(5M)-5-{8-[({4-[(propan-2-yl)oxy]phenyl}methyl)amino]quinolin-4-yl}pyridine-2-carbonitrile | 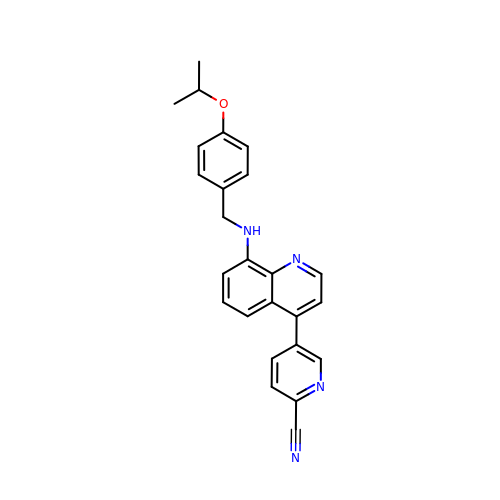C25 H22 N4 O | XKGFZUSEGLYHKC-UHFFFAOYSA-N> MEQNTTQVFSDLAYKVCFKVINDKNKPFVLHDEQRLANCLTRYVEAFNVT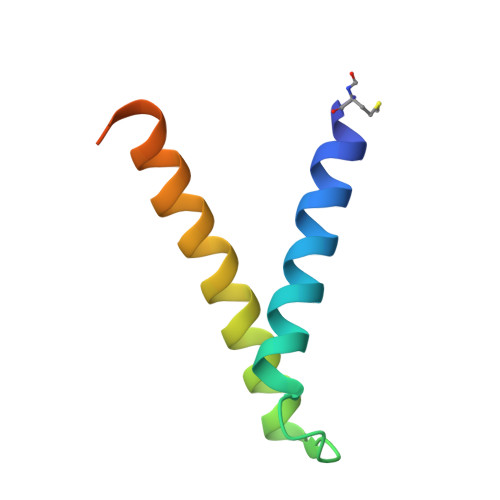SEYFFRERAGETKVTEKQ>[4x]AQCEATIESNDAMQYDLKEMVVDKSCKQFTVHLKHVGKMAKSAM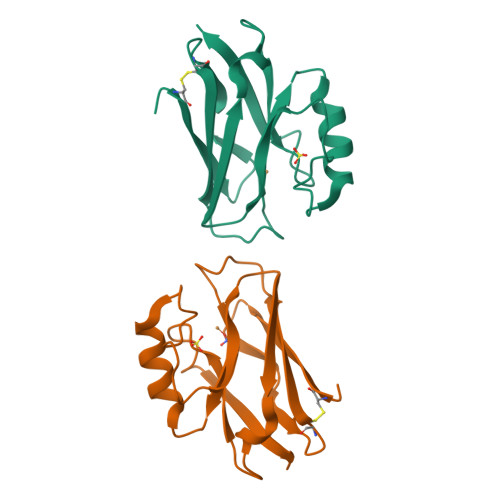GHNWVLTKEADKEGVATDGMNAGLAQDYVKAGDTRVIAHTKVIGGGESDSVTFDVSKLTPGEAYAYFCSFPGHWAMHKGTLKLSN> SPQPLEQIKLSESQLSGRVGMIEMDLASGRTLTAWRADERFPMMSTFKVVLCGAVLARVDAGDEQLERKIHYRQQDLVDYSPVSEKHLADGMTVGELCAAAITMGDNSA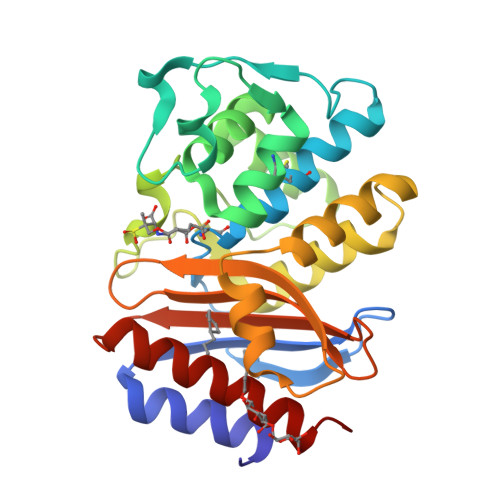ANLLLATVGGPAGLTAFLRQIGDNVTRLDRWETELNEALPGDARDTTTPASMAATLRKLLTSQRLSARSQRQLLQWMVDDRVAGPLIRSVLPAGWFIADKTGAGERGARGIVALLGPNNKAERIVVIYLRDTPASMAERNQQIAGIGAALIEHWQR> MSLHGKLIQFHKFGNPKDVLQVEYKNIEPLKDNEVFVRMLVRPINPSDLIPITGAYAHRIPLPNIPGYEGVGIVENVGAFVSRELIGKRVLPLRGEGTWQEYVKTSADFVVPIPDSIDDFTAAQMYINPLTAWVTCTETLNLQRNDVLLVNACGSAIGHLFAQLSQILNFRLIAVTRNNKHTEELLRLGAAYVIDTSTAPLYETVMELTNGIGADAAIDSIGGPDGNELAFSLRPNGHFLTIGLLSGIQVNWAEIVTKAKVHANIFHLRHWNDEVSPYKWQETFRHLIRLVENEQLRFMKVHSTYELADVKAAVDVVQSAEKTKGKVFLTSYEG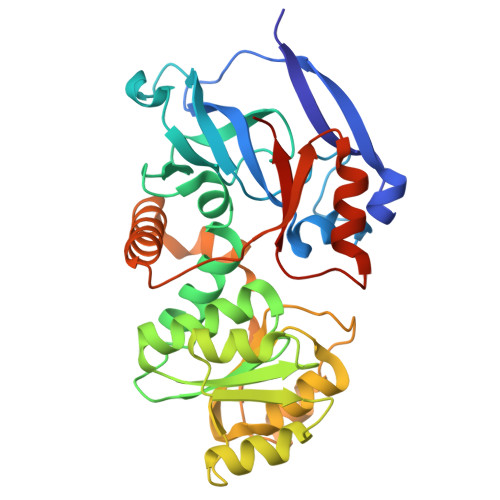HHHHHH> QNSVPHYAEADIVTLQGVTGGNTYAVPALPPG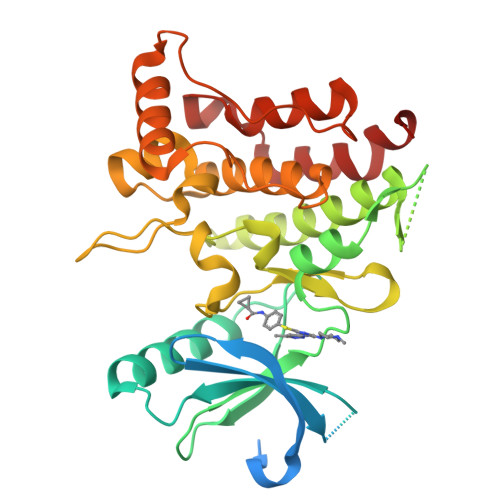AVGDGPPRVDFPRSRLRFKEKLGEGQFGEVHLCEVDSPQDLVSLDFPLNVRKGHPLLVAVKILRPDATKNARNDFLKEVKIMSRLKDPNIIRLLGVCVQDDPLCMITDYMENGDLNQFLSAHQLEDKAAEGAPGDGQAAQGPTISYPMLLHVAAQIASGMRYLATLNFVHRDLATRNCLVGENFTIKIADFGMSRNLYAGDYYRVQGRAVLPIRWMAWECILMGKFTTASDVWAFGVTLWEVLMLCRAQPFGQLTDEQVIENAGEFFRDQGRQVYLSRPPACPQGLYELMLRCWSRESEQRPPFSQLHRFLAEDALNTV>GSMAQILPIRFQEHLQLQNLGINPANIGFSTLTMESDKFICIREKVGEQAQVVIIDMNDPSNPIRRPISADSAIMNPASKVIALKAGKTLQ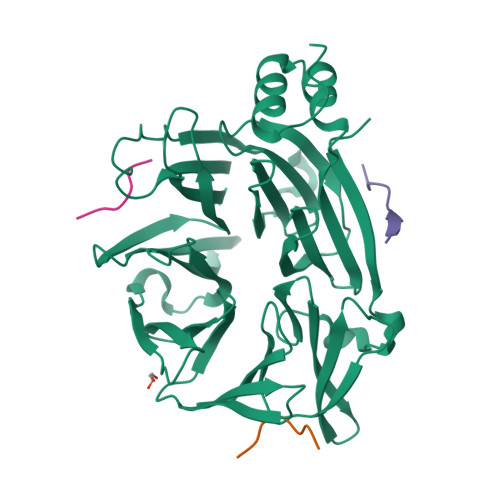IFNIEMKSKMKAHTMTDDVTFWKWISLNTVALVTDNAVYHWSMEGESQPVKMFDRHSSLAGCQIINYRTDAKQKWLLLTGISAQQNRVVGAMQLYSVDRKVSQPIEGHAASFAQFKMEGNAEESTLFCFAVRGQAGGKLHIIEVGTPPTGNQPFPKKAVDVFFPPEAQNDFPVAMQISEKHDVVFLITKYGYIHLYDLETGTCIYMNRISGETIFVTAPHEATAGIIGVNRKGQVLSVCVEEENIIPYITNVLQNPDLALRMAVRNNLAGAEEL[2x];>ETLLDLDFLE[6x]Rhizobium etli, a nitrogen-fixing bacterial symbiont of legume plants, encodes an essential l-asparaginase (ReAV) with no sequence homology to known enzymes with this activity. High-resolution crystal structures of ReAV show indeed a structurally distinct, dimeric enzyme, with some resemblance to glutaminases and β-lactamases. The active site of ReAV, deduced from structural comparisons and confirmed by mutagenesis experiments, contains a highly specific Zn2+ binding site without a catalytic role. There are two Ser-Lys tandems, all connected through a network of H-bonds to the Zn center, and three tightly bound water molecules near Ser48, which clearly indicate the catalytic nucleophile.

The orthorhombic (OP) and monoclinic MP1/MP2 forms show similar packing pattern with solvent content of 49.4–52.6%, whereas the monoclinic form MC, with a significantly different arrangement of the dimers in the unit cell, has 53.2% solvent content. In all cases the electron density maps have excellent definition for almost the entire protein molecules, except short disordered regions at the N- and C-termini. In the close vicinity of the Ser48 hydroxyl, there is a characteristic, almost tetrahedral pattern of three closely-spaced water molecules w2, w3, w4, visible in all crystal structures, except MP2. In all structures, regardless of the hydration state of Ser48, the side chain of Ser48 is also H-bonded to the Nζ atom of Lys51 and Oγ of Ser80.

>GIDPFTMTPSEDFVVTDRGGIVENSHRVHAAVVDAKGRLLYALGNPTRMTLARSAAKPAQALAILETEGVAGYGFDDADIALMCASHSSEDRHIARTRAMLSKIKAEEADLRCGGHPSLSEMVNRSWIKQDFIPTAVCSNCSGKHVGMLAGARAIGAGTDGYHLPDHPMQGRVKRTVAELCDLDAGDVEWGTDGCNLPTPAFPLDRLGRIYAKLASAADGSDAGEGQSTRCAALAHIFRAMARHPEMVAGEGRYCTMLMRAFDGALVGKLGADASYAIGVRASDATRQLGTDGALGISVKIEDGNLEMLYAVVTELLERLGIGSPDVRSQLASFHHPQRVNTMGVTTGGVSFPFKLRGSKSNVDDPRLAAVAR[4x]> SF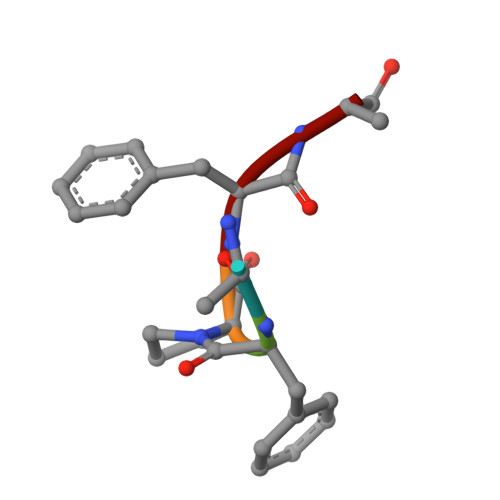PFT>GSKSSSSRRNAWGNLSYADLITKAIESSAEKRLTLSQIYEWMVKSVPYFKDKGDSNSSAGWKNSIRHNLSLHSKFIRVQNEGTGKSSWWMLNPEGGKSGKSPRRR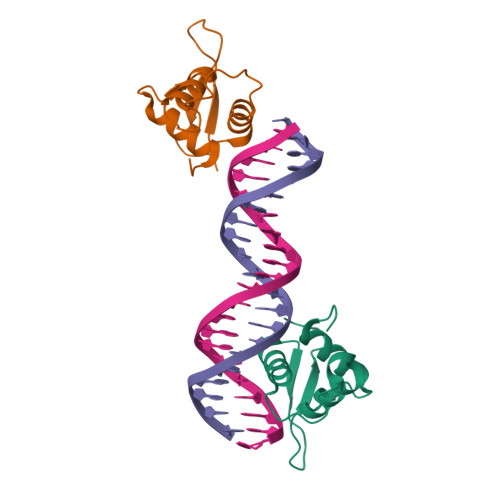AASMDN[2x]> MDDCRFETSELQASVMISTPLFTDSWSSCNTANCNGSIKIHDIAGITYVAIPAVSMIQLGNLVGLPVTGDVLFPGLSSDEPLPMVDAAILKLFLQLKIKEGLELELLGKKLVVITGHSTGGALAAFTALWLLSQSSPPSFRVFCITFGSPLLGNQSLSTSISRSRLAHNFCHVVSIHDLVPRSSNEQFWPFGTYLFCSDKGGVCLDNAGSVRL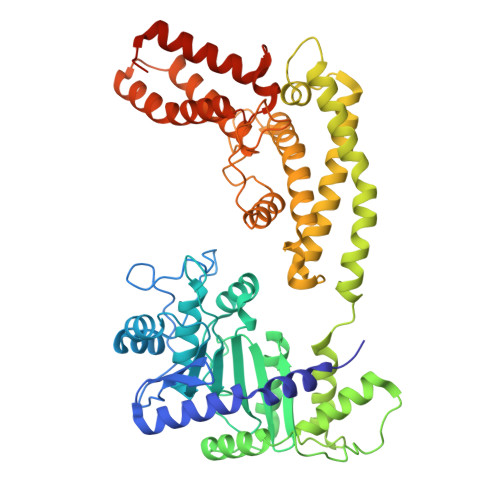MFNILNTTATQNTEEHQRYGHYVFTLSHMFLKSRSFLGGSIPDNSYQAGVALAVEALGFSNDDTSGVLVKECIETATRIVRAPILRSAELANELASVLPARLEIQWYKDRCDASEEQLGYYDFFKRYSLKRDFKVNMSRIRLAKFWDTVIKMVETNELPFDFHLGKKWIYASQFYQLLAEPLDIANFYKNRDIKTGGHYLEGNRPKRYEVIDKWQKGVKVPEECVRSRYASTTQDTCFWAKLEQAKEWLDEARKESSDPQRRSLLREKIVPFESYANTLVTKKEVSLDVKAKNSSYSVWEANLKEFKCKMGYENEIEMVVDESDAMET>[12x]MFKLSWIFGRKKDNAACSESAPEKVAQIPQHDPLDPMIKLGRIRGWNVEPEKAPVIRSVKDFLEPGLSVAMDSAYGDGPTPAAKAAAGGQNPYVVPTMLQDWYNSQGFIGYQACAIISQHWLVDKACSMSGEDAARNGWELKSDGRKLSDEQSALIARRDMEFRVKDNLVELNRFKNVFGVRIALFVVESDDPDYYEKPFNPDGITPGSYKGISQIDPYWAMPQLTAGSTADPSSEHFYEPDFWIISGKKYHRSHLVVVRGPQPPDILKPTYIFGGIPLTQRIYERVYAAERTAN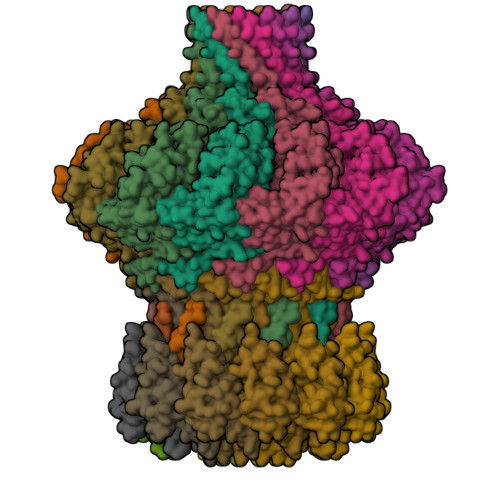EAPLLAMSKRTSTIHVDVEKAIANEDAFNARLAFWIANRDNHGVKVLGTDESMEQFDTNLADFDSIIMNQYQLVAAIAKTPATKLLGTSPKGFNATGEHETISYHEELESIQEHIFDPLLERHYLLLAKSEEIDVQLEIVWNPVDSTSSQQQAELNNKKAATDEIYINSGVVSPDEVRERLRDDPRSGYNRLTDDQAETEPGMSPENLAEFEKAGAQSAKAKGEAERAEAQAGAVEGAGDPVPAAPRGTKPLAKAAEEGASEAAEPPSRPDPKAELRNLLVDLLSKLQDLDDIKAPDGVDIEHNDAPGVKRTSKPGVSGMEPSVFSSNRIVGPRDHSELQRIKVNGITTLIENPRGSIRQGKDGSWRVQMKHHYGFIKGTKGADGDEVDCFVGPNLGSKRVFVVNQVNKEGQFDEHKCMLGFNNINDAKSGYLSCFRPGWDGLGSIHEVDLPAFRRWLANGDTTKPFGGE;>[12x]MVIFDEHKFRTLFPEFADPAAYPDVRLQMYFDIACEFISDRDSPYRILNGKALEACLYLLTAHLLSLSTMQVQGAAGGGVTAGGTQGGFITSATVGEVSVAKLAPPAKNGWQWWLSGTPYGQELWALLSVKAVGGFYIGGLPERRGFRKVGGTFW methyl beta-D-xylopyranoside | C6 H12 O5 | 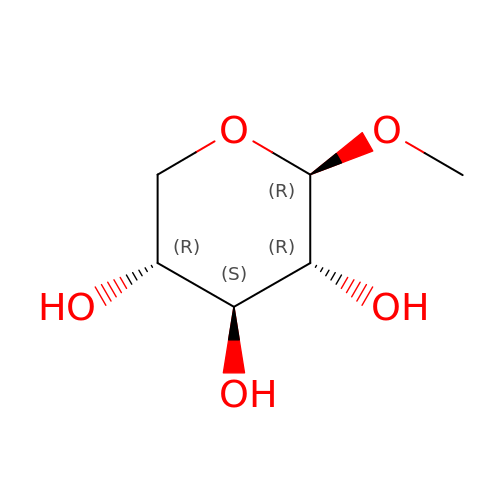ZBDGHWFPLXXWRD-JGWLITMVSA-N> QLRYSVVEESEPGTLVGNVAQDLGLKGTDLLSRRLRLGSEENGRYFSLSLVSGALAVSQKIDRESLCGASTSCLLPVQVVTEHPLELTRVEVEILDLNDNSPSFATPDREMRISESAAPGARFPLDSAQDPDVGTNTVSFYTLSPNSHFSLHVKTLKDGKLFPELVLEQQLDRETQARHQLVLTAVDGGTPARSGTSLIS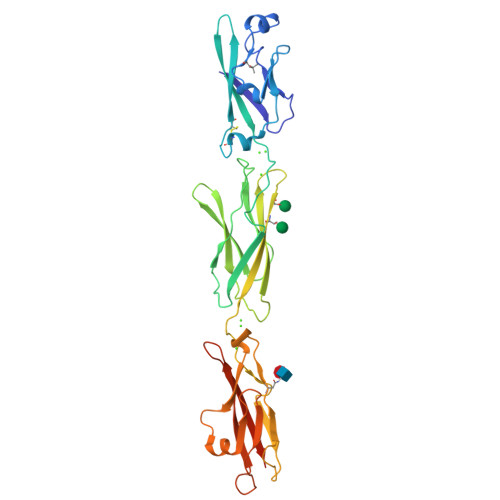VIVLDVNDNAPTFQSSVLRVGLPENTPPGTLLLRLNATDPDEGTNGQLDYSFGDHTSETVKNLFGLDPSSGAIHVLGPVDFEESNFYEIHARARDQGQPAMEGHCVIQVDVGDANDHHHHHHHH>MVTMEEIRKAQRAEGLATILAISTATPPNCVIQADYPDYYFKITNSEHMTELKEKFRRLCEKSMIRKRHMCLTEEILKANPNMCLHMGTSLNARQDISLVEVPKLGKEAATKAIKEWGQPKSKITHLIFCT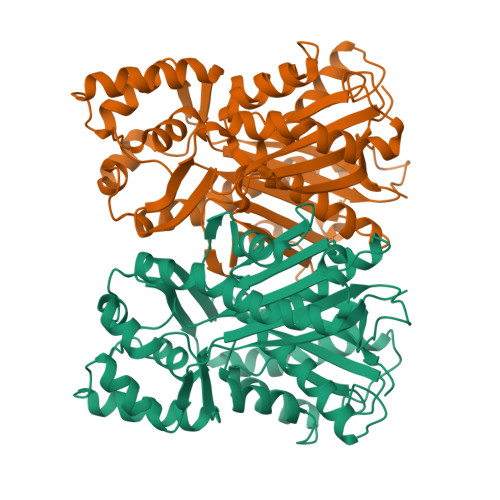SAGVDMPGADYQLTRLLGLSPEVKRMMIYQQGCYAGATVLRLAKDLTENNKGSRVLIVCSENTVPTFRGPSDTHIDSLVGQALFADGAAALIVGADPDASIERPLYHIVSASQTLLPDSDGAIEGHIREAGLTVHLKKDVPAFFSANIEKSLVDAFTPIGISDWNSIFWIAHPGGPAILDQVEEKLGLRKDKLKASRHVMSEFGNMSSACVLFILDEMRKTCLEEGKATTGEGLDWGVLFGFGPGLTVETVVLRSVPIEA[4x]> MGHHHHHHMLHLLEQIRAYCETCWEWQEAHEPGMDQDKNPMPAPVEHQICPAVCVLMKLSFDEEHRHAMNELGGLQAIAELLQVDCEMYG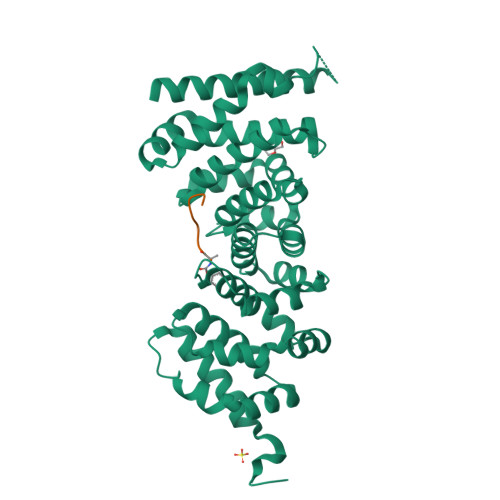LTNDHYSITLRRYAGMALTNLTFGDVANKATLCSMKGCMRALVAQLKSESEDLQQVIASVLRNLSWRADVNSKKTLREVGSVKALMECALEVKKESTLKSVLSALWNLSAHCTENKADICAVDGALAFLVGTLTYRSQTNTLAIIESGGGILRNVSSLIATNEDHRQILRENNCLQTLLQHLKSHSLTIVSNACGTLWNLSARNPKDQEALWDMGAVSMLKNLIHSKHKMIAMGSAAALRNLMANRPAKYKDANIMSPGSSLPS>[4x]VETISFSFSEFEPGNNDLTLQGAAI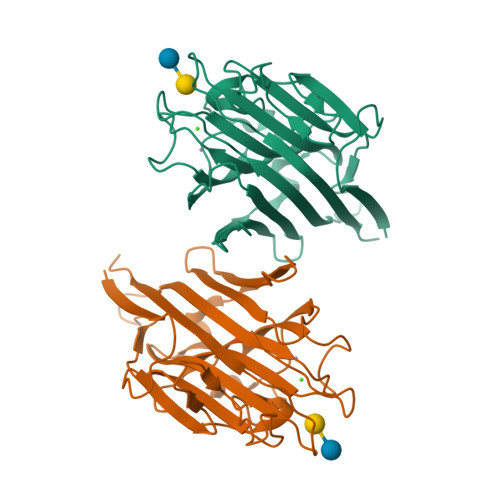ITQSGVLQLTKINQNGMPAWDSTGRTLYTKPVHIWDMTTGTVASFETRFSFSIEQPYTRPLPADGLVFFMGPTKSKPAQGYGYLGVFNNSKQDNSYQTLAVEFDTFSNPWDPPQVPHIGIDVNSIRSIKTQPFQLDNGQVANVVIKYDASSKILLAVLVYPSSGAIYTIAEIVDVKQVLPEWVDVGLSGATGAQRDAAETHDVYSWSFHASLPETND> MMPIKSIVTLDQLEDSEYLFRIVSTVLPHLCLDYKVCDQLKTTFVHPFDILLNNSLGSVTKQDELQAAISKLGINYLIDTTSRELKLFNVTLNAGNIDIINTPINISSETNPIINTHSFYDLPPFTQHLLNIRLTDTEYRARFIGGYIKPDGSDSMDVLAEKKYPDLNFDNTYLFNILYKDVINAPIKEFKAKIVNGVLSRQDFDNLIGVRQYITIQDRPRFDDAYNIADAARHYGVNLNTLPLPNVDLTTMPTYKHLIMFEQYFIYTYDRVDIYYNGNKMLFDDEIINFTISMRYQSLIPRLVDFFPDIPVNNNIVLHTRDPQNAAVNVTVALPNVQFVDINRNNKFFI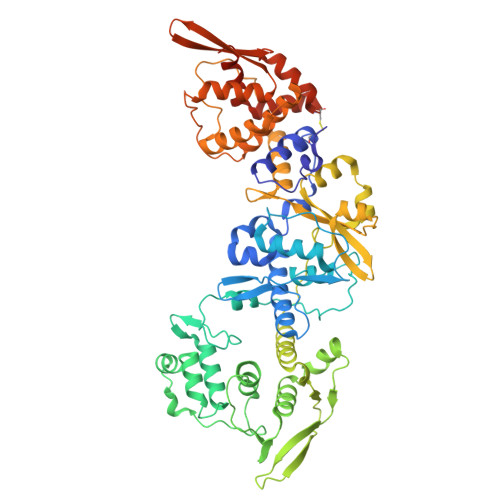NFFNLLAKEQRSTAIKVTKSMFWDGMDYEEYKSKNLQDMMFINSTCYVFGLYNHNNTTYCSILSDIISAEKTPIRVCLLPRVVGGKTVTNLISETLKSISSMTIREFPRKDKSIMHIGLSETGFMRFFQLLRLMADKPHETAIKEVVMAYVGIKLGDKGSPYYIRKESYQDFIYLLFASMGFKVTTRRSIMGSNNISIISIRPRVTKQYIVATLMKTSCSKNEAEKLITSAFDLLNFMVSVSDFRDYQSYRQYRNYCPRYFYAG>[2x]SNAMAWVVN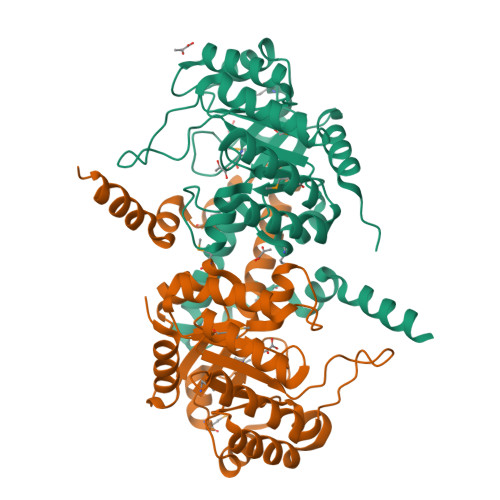KQSTQEELANRFRALVEANEILQIPGAHDAMAALVARNTGFLALYLSGAAYTASKGLPDLGIVTSTEVAERARDLVRATDLPVLVDIDTGFGGVLNVARTAVEMVEAKVAAVQIEDQQLPKKCGHLNGKKLVTTEELVQKIKAIKEVAPSLYIVARTDARGVEGLDEAIERANAYVKAGADAIFPEALQSEEEFRLFNSKVNAPLLANMTEFGKTPYYSAEEFANMGFQMVIYPVTSLRVAAKAYENVFTLIKETGSQKDALSNMQTRSELYETISYHDFEELDTGIAKTVLSEDQ> SSPGKPPRLVGGPMDASVEEEGVRRALDFAVGEYN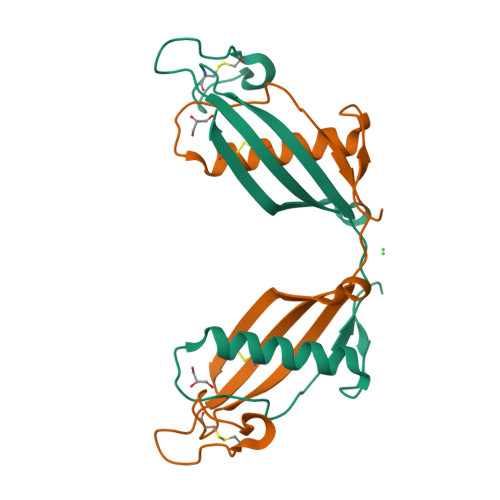KASNDMYHSRALQVVRARKQIVAGVNYFLDVELGRTTCTKTQPNLDNCPFHDQPHLKRKAFCSFQIYAVPWQGTMTLSKSTCQDA S-[(2E,6E)-3,7,11-TRIMETHYLDODECA-2,6,10-TRIENYL] 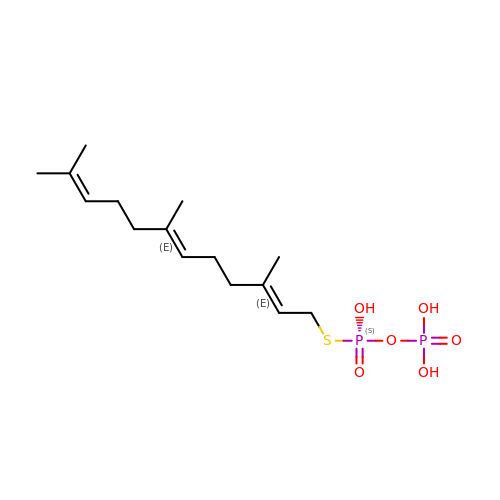TRIHYDROGEN THIODIPHOSPHATE | C15 H28 O6 P2 S | MYMLCRQRXFRQGP-YFVJMOTDSA-N>[2x]MAAPFEDLTNFERDNWNNWQAGPAGHDLYLVDASTRAVEFITRPNKNHAGEILKKTLTGLTAGYEYTWTVKIARIIG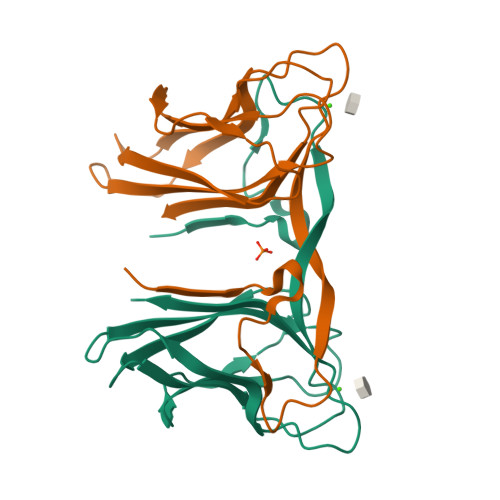KYEAPKVSLRADGKDISAPLELKQANEWVTLSGKFKATGSQAELAVVSHVSASMGNDFRIKELKIKG>[4x]AEQKTLHIY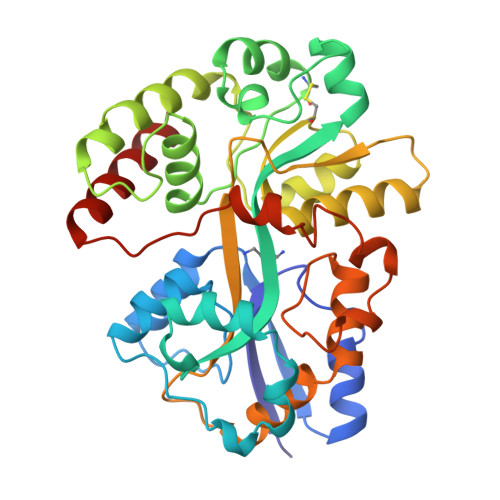NWSDYIAPDTVANFEKETGIKVVYDVFDSNEVLEGKLMAGSTGFDLVVPSASFLERQLTAGVFQPLDKSKLPEWKNLDPELLKLVAKHDPDNKFAMPYMWATTGIGYNVDKVKAVLGENAPVDSWDLILKPENLEKLKSCGVSFLDAPEEVFATVLNYLGKDPNSTKADDYTGPATDLLLKLRPNIRYFHSSQYINDLANGDICVAIGWAGDVWQASNRAKEAKNGVNVSFSIPKEGAMAFFDVFAMPADAKNKDEAYQFLNYLLRPDVVAHISDHVFYANANKAATPLVSAEVRENPGIYPPADVRAKLFTLKVQDPKIDRVRTRAWTKVKSGK> NAINPRLTPWTYRNTSFSSLPLTGENPGAWALVRDNSAKGITAGSGSQQTTYDPTRTEAALTASTTFALRRYDLAGRALYDLDFSKLNPQTPTRDQTGQITFNPFGGFGLSGAAPQQWNEVKNKVPVEVAQDPSNPYRFAVLLVPRSVVYYEQLQRGLGLPQQRTESGQNTSTTGAMFGLKVKNAEADTAKSNEKLQGAEATGSSTTSGSGQSTQRGGSSGDTKVKALKIEVKKKSDSEDNGQLQLEKNDLANAPIKRSEESGQSVQLKADDFGTALSSSGSGGNSNPGSPTPWRPWLATEQIHKDLPKWSASILILYDAPYARNRTAIDRVDHLDPKAMTANYPPSWRTPKWNHHGLWDWKARDVLLQTTGFFNPRRHPEWFDGGQTVADNEKTGFDVDNSENTKQGFQKEADSDKSAPIALPFEAYFANIGNLTWFGQALLVFGGNGHVTKSAHTAPLSIGVFRVRYNATGTSATVTGWPYALLFSGMVNKQTDGLKDLPFNNNRWFEYVPRMAVAGAKFVGRELVLAGTITMGDTATVPRLLYDELESNLNLVAQGQGLLREDLQLFTPYGWANRPDL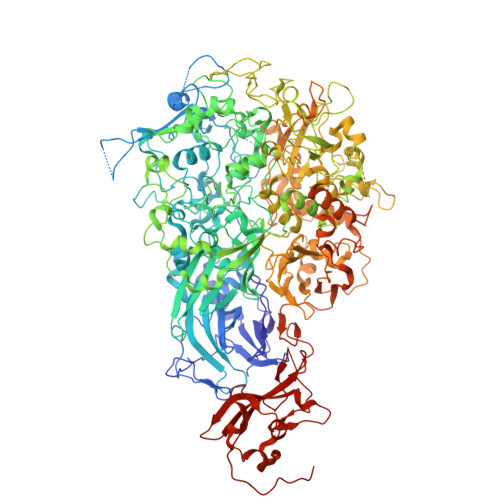PIGAWSSSSSSSHNAPYYFHNNPDWQDRPIQNVVDAFIKPWEDKNGKDDAKYIYPYRYSGMWAWQVYNWSNKLTDQPLSADFVNENAYQPNSLFAAILNPELLAALPDKVKYGKENEFAANEYERFNQKLTVAPTQGTNWSHFSPTLSRFSTGFNLVGSVLDQVLDYVPWIGNGYRYGNNHRGVDDITAPQTSAGSSSGISTNTSGSRSFLPTFSNIGVGLKANVQATLGGSQTMITGGSPRRTLDQANLQLWTGAGWRNDKASSGQSDENHTKFTSATGMDQQGQSGTSAGNPDSLKQDNISKSGDSLTTQDGNAIDQQEATNYTNLPPNLTPTADWPNALSFTNKNNAQRAQLFLRGLLGSIPVLVNRSGSDSNKFQATDQKWSYTDLHSDQTKLNLPAYGEVNGLLNPALVETYFGNTRAGGSGSNTTSSPGIGFKIPEQNNDSKATLITPGLAWTPQDVGNLVVSGTTVSFQLGGWLVTFTDFVKPRAGYLGLQLTGLDASDATQRALIWAPRPWAAFRGSWVNRLGRVESVWDLKGVWADQAQSDSQGSTTTATRNALPEHPNALAFQVSVVEASAYKPNTSSGQTQSTNSSPYLHLVKPKKVTQSDKLDDDLKNLLDPNQVRTKLRQSFGTDHSTQPQPQSLKTTTPVFGTSSGNLSSVLSGGGAGGGSSGSGQSGVDLSPVEKVSGWLVGQLPSTSDGNTSSTNNLAPNTNTGNDVVGVGRLSESNAAKMNDDVDGIVRTPLAELLDGEGQTADTGPQSVKFKSPDQIDFNRLFTHPVTDLFDPVTMLVYDQYIPLFIDIPASVNPKMVRLKVLSFDTNEQSLGLRLEFFKPDQDTQPNNNVQVNPNNGDFLPLLTASSQGPQTLFSPFNQWPDKHHHHHH> MSAKKIVLKSSDGESFEVEEAVALESQTIAHMVEDDCVDNGVPLPNVTSKILAKVIEYCKRHVEAAASKAEAVEGAATSDDDLKAWDADFMKIDQATLFELILAANYLNIKNLLDLTCQTVADMIKG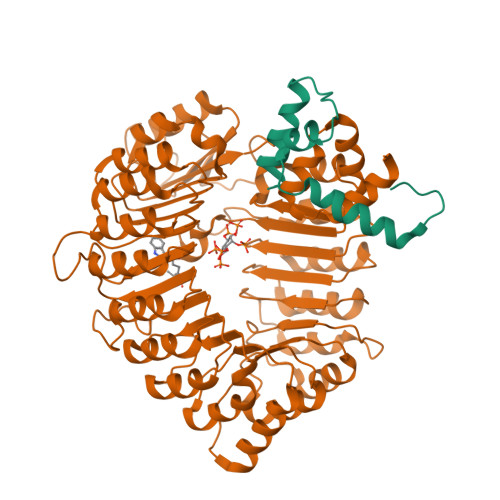KTPEEIRTTFNIKNDFTPEEEEEVRRENQWAFE;> MQKRIALSFPEEVLEHVFSFIQLDKDRNSVSLVCKSWYEIERWCRRKVFIGNCYAVSPATVIRRFPKVRSVELKGKPHFADFNLVPDGWGGYVYPWIEAMSSSYTWLEEIRLKRMVVTDDCLELIAKSFKNFKVLVLSSCEGFSTDGLAAIAATCRNLKELDLRESDVDDVSGHWLSHFPDTYTSLVSLNISCLASEVSFSALERLVTRCPNLKSLKLNRAVPLEKLATLLQRAPQLEELGTGGYTAEVRPDVYSGLSVALSGCKELRCLSGFWDAVPAYLPAVYSVCSRLTTLNLSYATVQSYDLVKLLCQCPKLQRLWVLDYIEDAGLEVLASTCKDLRELRVFPSEPFVMEPNVALTEQGLVSVSMGCPKLESVLYFCRQMTNAALITIARNRPNMTRFRLCIIEPKAPDYLTLEPLDIGFGAIVEHCKDLRRLSLSGLLTDKVFEYIGTYAKKMEMLSVAFAGDSDLGMHHVLSGCDSLRKLEIRDCPFGDKALLANASKLETMRSLWMSSCSVSFGACKLLGQKMPKLNVEVIDERGAPDSRPESCPVERVFIYRTVAGPRFDMPGFVWNMDQDSTMRFSRQIITTNGL>[2x]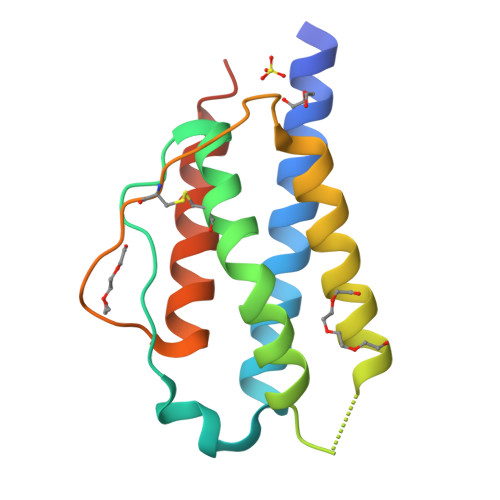APTTSSSTKEAQQQLEQLLLDLQLLLNGVKNYESPRMLTFKFYMPKKATELTHLQCLAEELKLLEEVLYLAQSKNFHLTDIKELMSNINVTLLKLKGSETSFKCEYDDETVTITEFLNKWITFCQSIFSTLTHHHHHH>[6x]SASFDGPKFKMTDGSYVQTKTIDVGS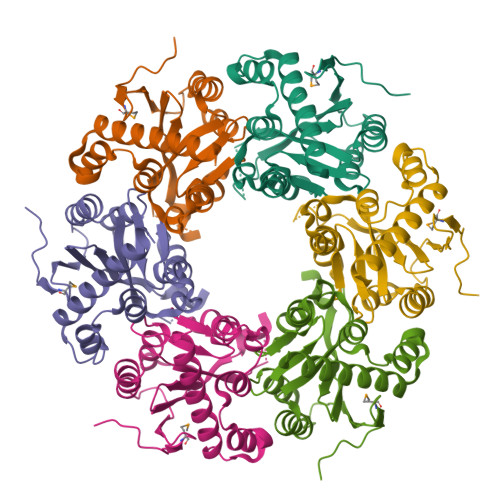STDISPYLSLIREDSILNGNRAVIFDVYWDVGFPETETKTKTSGWSLSSVKLSTRNLCLFLRLPKPFHDNLKDLYRFFASKFVTFVGVQIEEDLDLLRENHGLVIRNAINVGKLAAEARGTLVLEFLGTRELAHRVLWSDLGQLDSIEAKWEKAGPEEQLEAAAIEGWLIVNVWDQLSDE Integrins are widely expressed cell surface receptors that couple cell- extracellular matrix (ECM) interactions with the cytoskeleton and transduce mechanochemical signals across the plasma membrane initiating a biological response. Four I domain-containing integrins (α1β1, α2β1, α10β1, and α11β1) function as collagen receptors on numerous cell types. The bond consists of a glutamate or aspartate in the ligand and a metal ion bound by a metal ion dependent adhesion site (MIDAS) within the I domain. In contrast, while Ca2+ promotes α1I ligand binding, it inhibits α2I binding, suggesting these ions differentially regulate the interaction of integrins with their cognate ligands.

The α1I asymmetric unit comprises two molecules whose structures were analyzed for discrepancies relevant to Ca2+ binding. The RMSD between the A and B α1I molecules is 0.13 Å. More specifically, the α1I domain Ca2+ coordinates D253, S152 and S154. D150 and T220 interactions with Ca2+ are water-mediated (ω1). In total, the Ca2+ is heptacoordinated with three residues and four water molecules. The metal-I domain side chain bond distances are approximately 2.4 Å. Exclusive alignment of Ca2+ vs. Mg2+-bound α1I MIDAS residues produced a RMSD of 0.24 Å. We found that Ca2+ functionally substitutes for Mg2+ in the α1I structure. Specifically, Ca2+ is properly positioned in α1I to facilitate binding by coordination with an acidic ligand side chain, initiating the allosteric mechanism that leads to signal transduction. Specifically, increased flexibility in α1I domain loops βB-βC and α3-α4 would allow for the expansion of the MIDAS pocket necessary to bind the larger Ca2+ ion.

>QLDIVIVLDGSNSIYPWDSVTAFLNDLLERMDIGPKQTQVGIVQYGENVTHEFNLNKYSSTEEVLVAAKKIVQRGGRQTMTALGIDTARKEAFTEARGARRGVKKVMVIVTDGESHDNHRLKKVIQDCEDENIQRFSIAILGSYNRGNLSTEKFVEEIKSIASEPTEKHFFNVSDELALVTIVKTLGERIFALEA[2x]>[4x]CGGACCGAGCCAG;>GCUGGG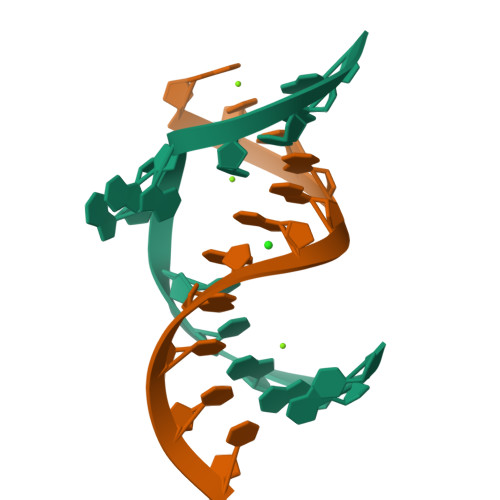AGUCC[4x]Especially, exposure or modification of N-terminal amino acid residues can mediate protein degradation and the resultant proteolytic procedure is called the N-degron pathway (formerly the N-end rule pathway). Two tertiary degrons, Asn and Gln, are hydrolyzed into the secondary degron Asp and Glu by N-terminal asparagine amidohydrolase 1 (NTAN1) and N-terminal glutamine amidohydrolase 1 (NTAQ1), respectively. In multicellular eukaryotes, Nt-Asn and Nt-Gln are deamidated by NTAN1-encoded NtN-amidase and NTAQ1-encoded NtQ-amidase, respectively. In this study, the crystal structure of NTAN1, the last veiled structure among three amidases in the N-degron pathway, was elucidated.

Although yNta1, NTAQ1, and NTAN1 do appear to share catalytic functions commonly involving a conserved Cys residue critical for the deamidation activity, they exhibit low sequence similarity to each other. And we explain unexpected substrate specificities of NTAN1 based on structural and biochemical analyses.

>MPLLVEGRRVRLPQSAGDLVRAHPPLEERARLLRGQSVQQVGPQGLLYVQQRELAVTSPKDGSISILGSDDATTSHIVVLRHTGNGATCLTHCDGTDTKAEVPLIMNSIKSFSDHAQCGRLEVHLVGGFSDDRQLSQKLTHQLLSEFDRQEDDIHLVTLCVTELNDREENENHFPVIYGIAVNIKTAEIYRASFQDRGPEEQLRAARTLAGGPMISIYDAETEQLRIGPYSWTPFPHVDFWLHQDDKQILENLSTSPLAEPPHFVEHIRSTLMFLKKHPSPAHTLFSGNKALLYKKNEDGLWEKISSPGSLEHHHHHH[2x];>[2x]NFAAR(1S,2S)-N-[4-(phenylsulfonyl)phenyl]-2-(pyridin-3-yl)cyclopropanecarboxamide 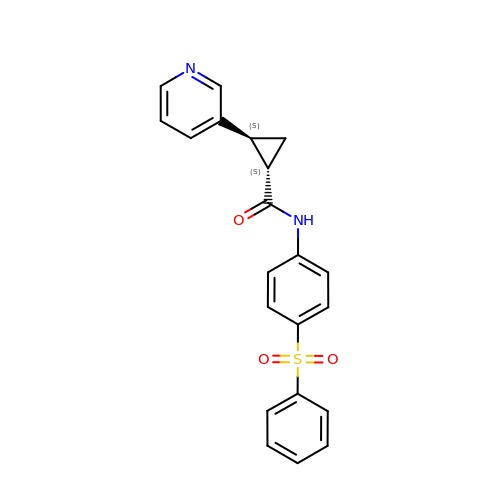| C21 H18 N2 O3 S | YERMBKYNILMCNC-UXHICEINSA-N> SWQAYTDNLIGTGKVDKAVIYSRAGDAVWATSGGLSLQPNEIGEIVQGFDNPAGLQSNGLHIQGQKFMLLRADDRSIYGRH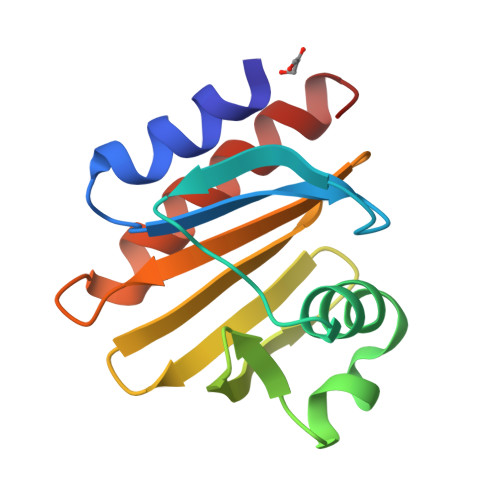DAEGVVCVRTKQTVIIAHYPPTVQAGEATKIVEQLADYLIGVQY> MELSASATELLQDYMLTLRTKLSSQEIQQFAALLHEYRNGASIHEFCINLRQLYGDSRKFLLLGLRPFIPEKDSQHFENFLETIGVKDLEHHHHHH;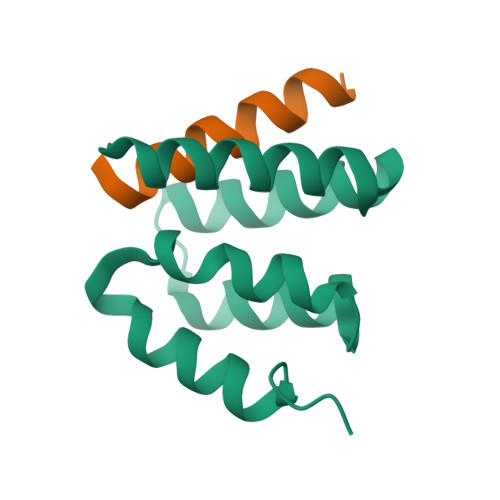> MDEQEALNSIMNDLVALQMNRR(2S)-2-amino-4-(S-butylsulfonimidoyl)butanoic acid | C8 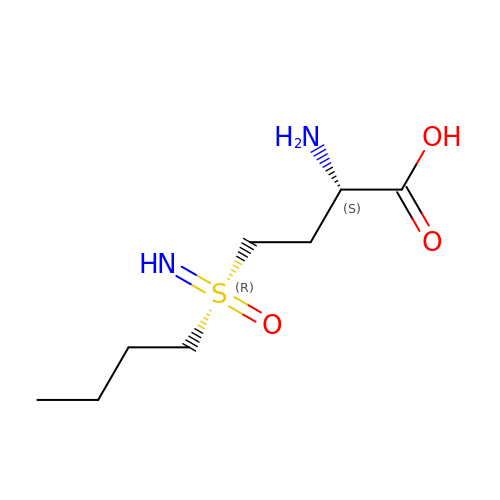H18 N2 O3 S | KJQFBVYMGADDTQ-JKYUHCHBSA-N2-{(3S)-3-[(benzylsulfonyl)amino]-2-oxopiperidin-1-yl}-N-{(2S)-1-[(3R)-1-carbamimidoylpiperidin-3-yl]-3-oxopropan-2-yl}acetamide 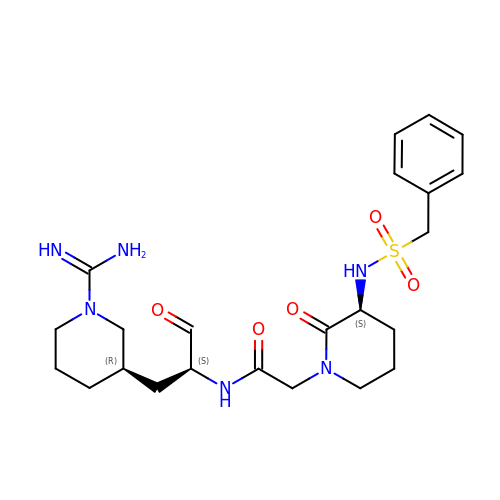| C23 H34 N6 O5 S | DATYERRDSFNBDN-AABGKKOBSA-N>MASDKFPVAENPSSSFKYESAVQYRPAPDSYLNPCPQAGRIVKETYTGINGTKSLNVYLPYGYDPNKKYNIFYLMHGGGENENTIFSNDVKLQNILDHAIMNGELEPLIVVTPTFNGGN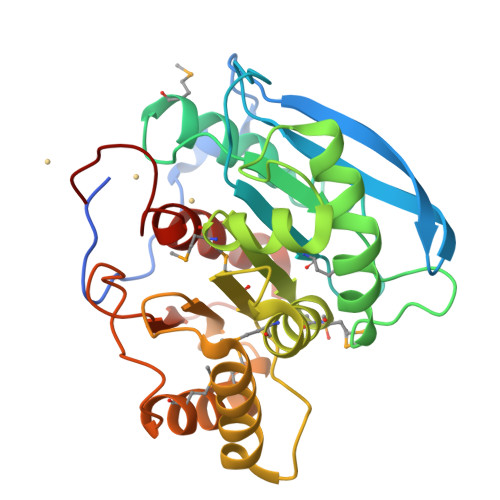CTAQNFYQEFRQNVIPFVESKYSTYAESTTPQGIAASRMHRGFGGFSMGGLTTWYVMVNCLDYVAYFMPLSGDYWYGNSPQDKANSIAEAINRSGLSKREYFVFAATGSEDIAYANMNPQIEAMKALPHFDYTSDFSKGNFYFLVAPGATHWWGYVRHYIYDALPYFFHELEHHHHHH[2x]> RGSHGGSMGPQVVKVEDIDFATKFTPPTGSTELDLIGYGNTGMEIETVEIRFTAIGFYAEPSISEHLQKWKGTPSSNLVEDDSGFHKELIQAPVEKAVRISIIKGIKGLPYGSALQSSLRDRLVNNDLFEEEEEEALEKLAEFFQPHNLPKGTNIIYHWATPSSVKV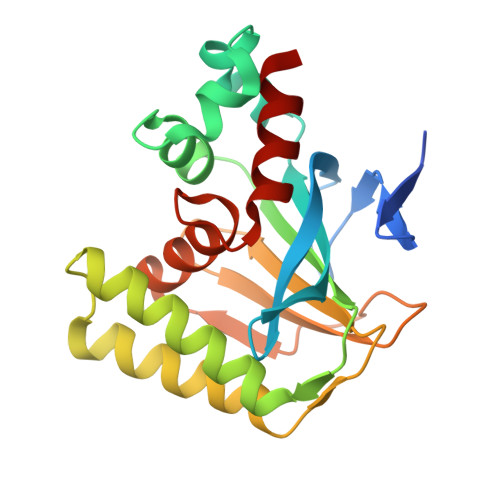SLSEEGKMPEDVAYTIDDAHVAEALLDLYLGENTITPSTLASVAEAIAA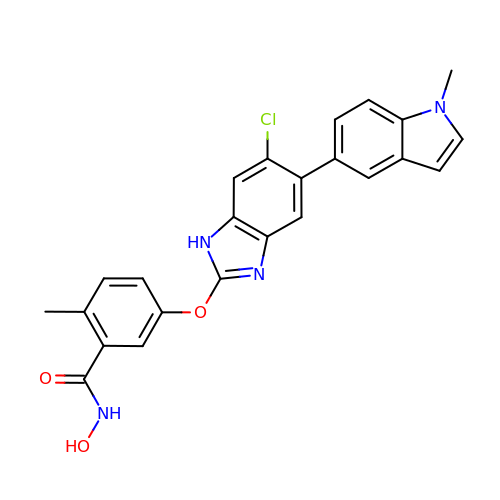5-{[6-chloro-5-(1-methyl-1H-indol-5-yl)-1H-benzimidazol-2-yl]oxy}-N-hydroxy-2-methylbenzamide | C24 H19 Cl N4 O3 | SCEVBRBKKQZTKM-UHFFFAOYSA-N> MISYEFQTHLPKGKDSSLNASSENKELYVQATHFNNTILLQIRLNGEMDSTYEVSSKGLNPILDINVPLAGNLGNTGGDYDDEEEEFVRDHLSDYQVVTKLGDSADPKVPVVCVQIAELYRRVILPEVSGTM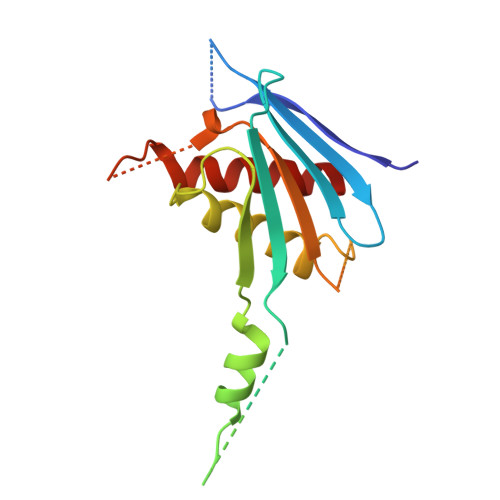AQDNMQFSLLISMSSKIWRATKEQSADDNDFGKLVFVLKCIKDMYAK> VHHPPSYVAHLASDFGVRVFQQVAQASKDRNVVFSPYGVASVLAMLQLTTGGETQQQIQAAMGFKIDDKGMAPALRHLYKELMGPWNKDEISTTDAIFVQRDLKLVQGFMPHFFRLFRSTVKQVDFSEVERARFIINDWVKTHTKGMISNLLGKGAVDQLTRLVLVNALYFNGCWKTPFPDSSTHRRLFHKSDGSTVSVPMMAQTNKF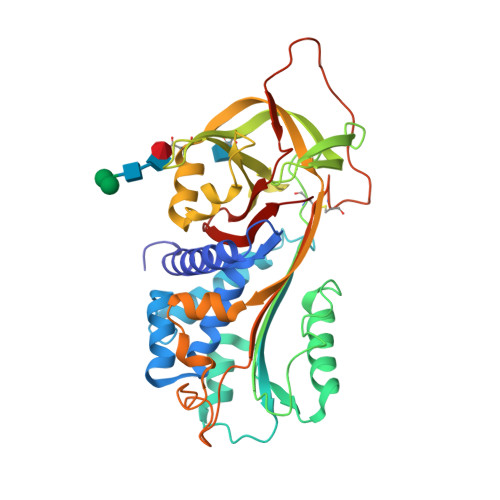NYTEFTTPDGHYYDILELPYHGDTLSMFIAAPYEKEVPLSALTNILSAQLISHWKGNMTRLPRLLVLPKFSLETEVDLRKPLENLGMTDMFRQFQADFTSLSDQEPLHVAQALQKVKIEVNESCTVASSSTAVIVSARMAPEEIIMDRPFLFVVRHNPTGTVLFMGQVMEP>GSHMASNDLIYQDEHASLQPLEGRTVAVIGYGIQGRAFAANLRDSGVAVRVGNIDDRYFELARAEGHRVTNIAEAVAHADIVLLLIPDEAHGAVFDVDIAPNLRDGALLCVAHGHSLVQGDVRPLPGRDLAMLAPRMYGDPIRRYYLAGQGAPAYFDIVADHTGRARDRVLAIARAVGFTRAGVMALGYRQETFLDLFQEQFLAPALVDLVETGFQVLVERGFNPKAALLEVYGSGEMGKMMLDGADIGLDEVVALQGSPTCQVGYHRWRGRTLPTAVRELAARVLDQIEGGDFSAYLKEQASNDYASLDDARRAALKRPLNVAHAQVRAAFRFPTEAAGGLYQAAQAPADVEPEA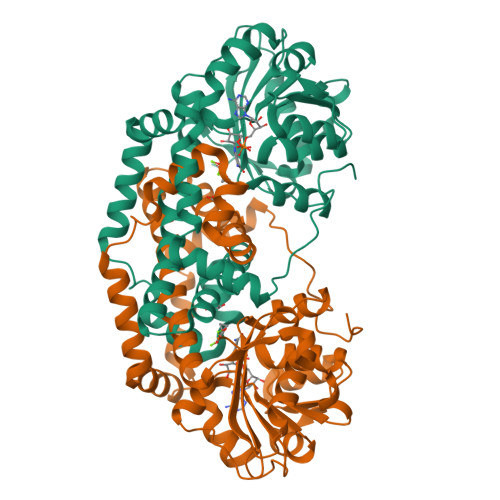AR[2x]> MIRTTNTCCGNQAGMVEKFIGTAYDVVKTVYDNLGEIQFIYNFLNDYGVLITVDSVTELQELPTTAKYTRVYSSTPTGVRIYTDYLYVEGDRTGVLPSDPTATGSWVVVGSSNSGAATGTGAYIPFVFNNGSAAGGETTIVVPDYTI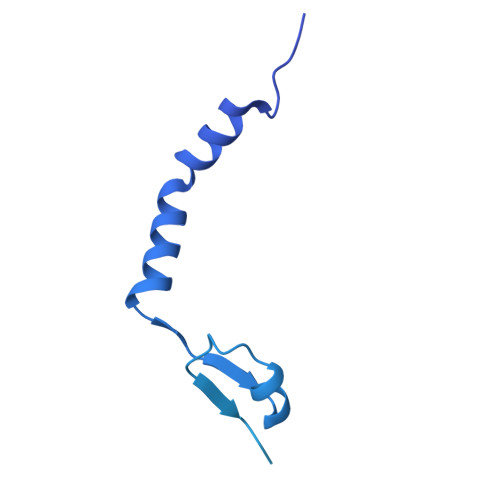GVPEIYVEGFRQQVGRGFTFNSVNLTVTLAQPLEQGDEVVLMLSGNPAVPDNPNIDSWTVINWIYNNGAAVGGEQVIVIPYTFQTVPAIFKNGLRYQGGLSTQSYTVDQDNKRILLTEPLSTNDRLVVQLGGELVTLESPDRSLYEIARATNMKDSEVIKSDNTVETLNGKRILYDIVSQVYYWIPSSVPNNVYIQSVVNGQLTYLPGNIVVTLTPIVTLGLSGTTAQRPIGVLTGTQHFDTTLGKPIWFNGTAWVDSTGAVV> GPHMPPSERAEKQAAAQQAVDILHEIATILNCHLDRRTLSICISMIENGVNPEALANVIKELR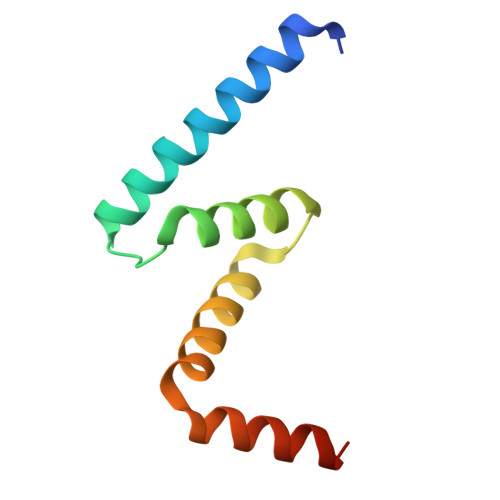VLGQDPQQLDALVANYLASSRRR> MEELQKSIGHKPEPTDEEWELIKTVTEAHVATNAQGSHWKQKRKFLPEDIGQAPIVNAPEGG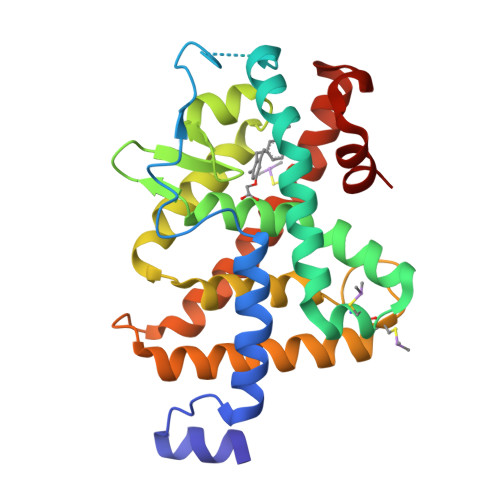KVDLEAFSHFTKIITPAITRVVDFAKKLPMFCELPCEDQIILLKGCCMEIMSLRAAVRYDPESETLTLNGEMAVTRGQLKNGGLGVVSDAIFDLGMSLSSFNLDDTEVALLQAVLLMSSDRPGLACVERIEKYQDSFLLAFEHYINYRKHHVTHFWPKLLMKVTDLRMIGACHASRFLHMKVECPTELFPPLFLEVFED>[2x]TYTTRQIGAKNTLE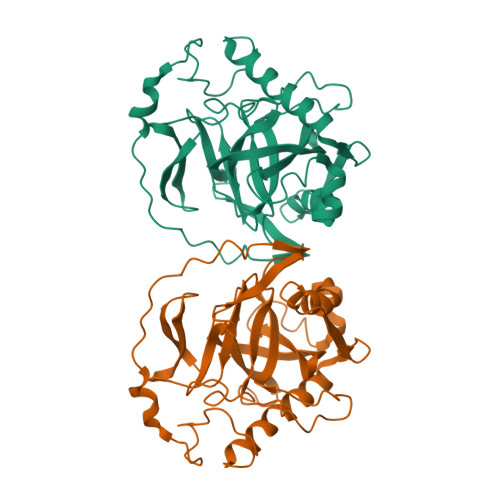YKVYIEKDGKPVSAFHDIPLYADKEDNIFNMVVEIPRWTNAKLEITKEETLNPIIQNTKGKLRFVRNCFPHHGYIHNYGAFPQTWEDPNVSHPETKAVGDNNPIDVLQIGETIAYTGQVKEVKALGIMALLDEGETDWKVIAIDINDPLAPKLNDIEDVEKYFPGLLRATDEWFRIYKIPDGKPENQFAFSGEAKNKKYALDIIKETHNSWKQLIAGKSSDSKGIDLTNVTLPDTPTYSKAASDAIPPASPKADAPIDKSIDKWFFISGSV> MEITGPHTNTVIEWSNLINTNTWLLYQKPLNSVRLLKHGPDTYNSNLAAFELWYGKSGTTITSVYYNTINNQNKTHDANSDCLILFWNEGSTQLE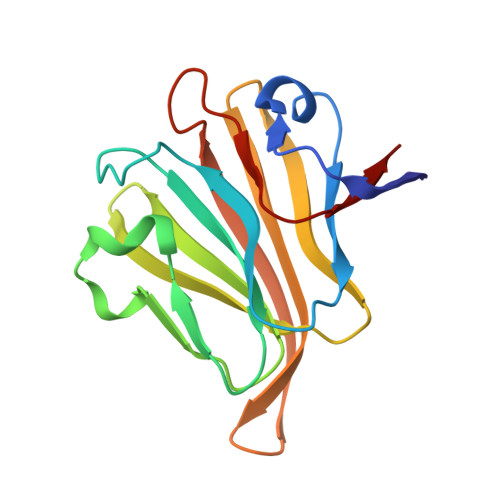KQVVTFNWNVGGILIKPINSSRMRICMSGMENFNNDSFNWENWNHEFPRSNPGININMYTEYFLASS> MILSDKDIIDYVTSKRIIIKPFNKDFVGPCSYDVTLGDEFIIYDDEVYDLSKELNYKRIKIKNSILVCPLNYNLTEEKINYFKEKYNVDYVVEGGVLGTTNEYIELPNDISAQYQGRSSLG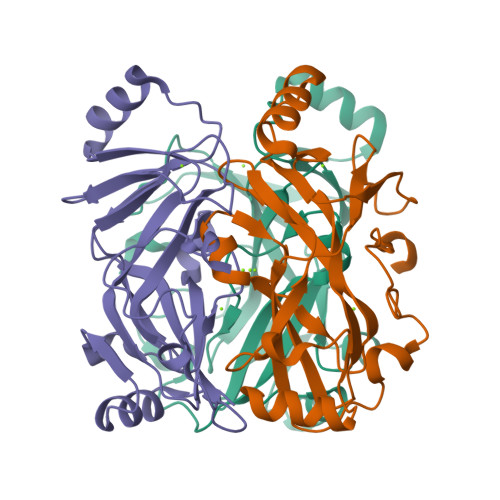RVFLTSHQTAGWIDAGFKGKITLQIVAFDKPVILYKNQRIGQLIFSKLLSPADVGYSERKTSKYAYQKSVMPSLIHLDNHKKD>[2x]MLDTNMKTQLRAYLEKLTKPVELIATLDDSA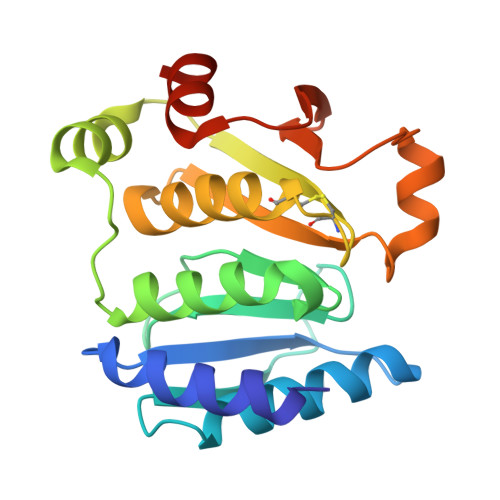KSAEIKELLAEIAELSDKVTFKEDNTLPVRKPSFLITNPGSQQGPRFAGSPLGHEFTSLVLALLWTGGHPSKEAQSLLEQIRDIDGDFEFETYYSLSCHNCPDVVQALNLMAVLNPRIKHTAIDGGTFQNEITERNVMGVPAVFVNGKEFGQGRMTLTEIVAKVDTGAEKR>MKLAVAALLVASAAAFAPAPASKASTSLKVSEIELGVTEPLGVYDPLGWLESEPEAFERRRAVERKHGRVAMAAVVGTIVHNNHIVFDGYLSPSNNLKFSDIPTGVDGIRAIPTAGLAQILAFFALVELAWMPASKYDGDYGVGYFGTDIKDPEEKARKLNVELNNGRAAMMGIMGNMVAEVLTGQTMYEQYASGHISPFGDGQGVF[5x];> MKLAIAALLCASAAAFAPAPASKVSTALNVNELEIGATAPLGVYDPLGWLDGEPENFERRRAVERKHGRVAMAAVVGTIVHNNHITFDGYLSPSANLKFSDIPTGVDGIRAIPTAGLLQILFFFALVELAWMPASKYDGDYGVGWFGSNIEDPEEKARKLNVELNNGRAAMMGIMGNMVTECITGQTMYEQYAAGHFSPFGDGQGAF;> MKTAILAAMLGSAAAFVPAQQSKVSTSLAASELEDGIGAVAPLGYFDPLGYIKDEETFIRYRAVERKHGRVAMMAMLGTFVHNNGWTFDGYLSPSQGLKFSDIDSGIGGLFQVPPAGLAQIILLCGFVELAWWPASNLSGDYGVRLGTLNDWEEQPAKYYRQKNAELNNGRAAMMGILGTFTHEVITGQNFAEQAAAGHFSPFGDGQGFF;> MKLAIAALLATSAAAFTTSPASRATTSLQVSEIELGATEPLGVFDPLGWLETEPEAFERRRAVERKHGRVAMAAVVGTIVHNNHIVFDGYISPSNNLKFSDIPTGIDGIFSVPTAGLAQIIAFLGFVELAWLPASQYDGDYGVGYFGNDILDPEEKARKLNAELNNGRAAMMGIMGNMVAEKITGQTMYEQYAAGHFNPFNDGEGFF;> MKLALAALLATSAAAFQAPTMTFSLGKKAAAKKAVKAPAPSGASPSADAWANSIESKALPFARAPATLDGTMLGDFGFDPLGFSTVPVGPWFTGIEGRNGQIGNLNWYREAELIHGRIAQVAVVGFIAPGLFGTLPGNEWTGVDAYSNLNPLEAFSQVPGLAILQIFLFMSYLEVRRINIIKEEGENYMPGDLRIGQGEGRWNPFGLDYSPEAYEEKRLQELKHCRLAMIGVFGLWAQAQASGVGVTEQIGAALTTPDYYAKAGYFLPEGI;> MKSIAALLALASAAAAFTPQSQSTSSTALKE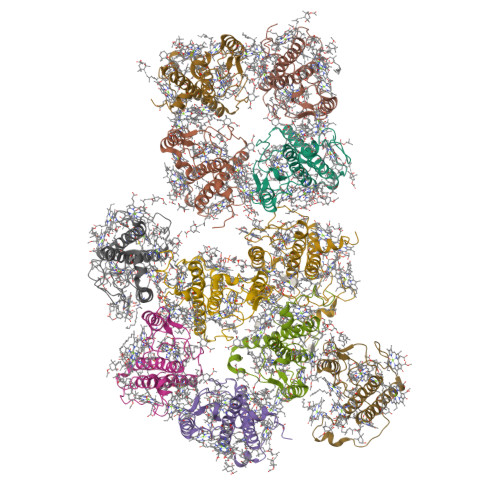RISPLDPSIGVTEPLGLYDPLGWLDPEKDPASKFATFHANFERRRAVERKHGRIAMVAVVGMLFHNADIEFPGYLSKELGIRFSDVPNGMNGLFSIPLAGLTQIVFAIGVMELAIWPASNYSGDYGTGYGRPFVPNVLEGDELKYKLDMEINQGRAAMMGIMGALVGEAVTGQTLAEQIASNNLGLFSALFE;> MKLALLASLVASAAAFAPSKVAQTSTALKAFENELGAQPPLGFFDPLGLVEDGNQAKFDRLRYVELKHGRISMLAVVGYLIEKAGIRLPGNISYDGTSFADIPDGFAALSKIPDAGLFQLFAFIGFLEVFVMKDITGGEFVGDFRNGFIDFGWDSFDEETKLKKRAIELNQGRAAMMGILALMVHEKLGVSLLPQ> METTYKLLDGKKISGEIKQEIAAVVNELLEKGGRRPHLAGVLVGHDGGSETYMASKVKACEEVGFTSSLIRYEDDVTEEELLACVHRLNQDPTVDGFIVQLPLPKHIDEQKIIEAVDPRKDVDGFHPINVGRLSIGL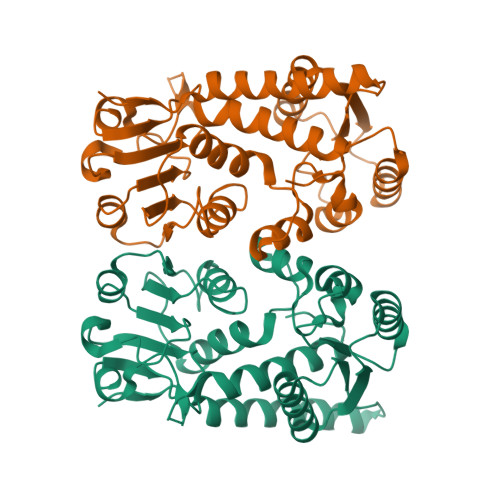PGFVSATPKGIVELLRRYNIPTRGKHCVVLGRSNIVGKPVSQLLLQKGEPGDCTITICHSRTPNIKEVCLTADIIIAALGQPEFLTADMVKPGAVVVDVGTTLVPDSTRKSGFRLTGDVKFDEVAPKCSYITPVPGGVGPMTIVSLMSNTLLASKGLYR>SQPDPKPDELHKSSKFTGLMEAMKVLYDDNHVSAINVKSIDQFLYFDLIYSIKDTKLGNYDNVRVEFKNKDLADKYKDKYVDVFGANYAYQCYFSKKTNDINSHQTDKAKTCMYGGVTEHNGNQLDKYRSITVRVFEDGKN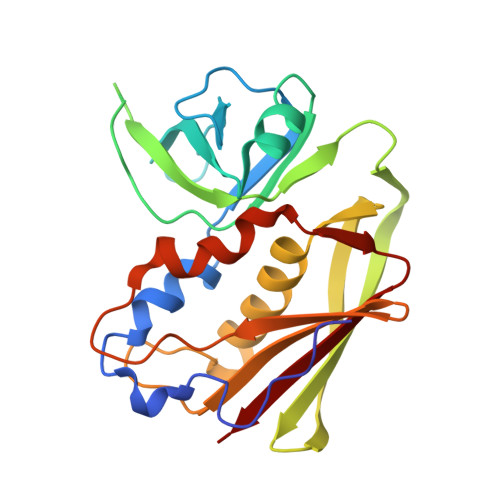LLSFDVQTNKKKVTAQELDYLTRHYLVKNKKLYEANNSPYETGYIKFIENENSFWYDMMPAPGDKFDQSKYLMMYNDNKMVDSKDVKIEVYLTT[2x]N-({4-[(2-amino-6-ethyl-4-oxo-3,4-dihydrothieno[2,3-d]pyrimidin-5-yl)sulfanyl]phenyl}carbonyl)-L-glutamic 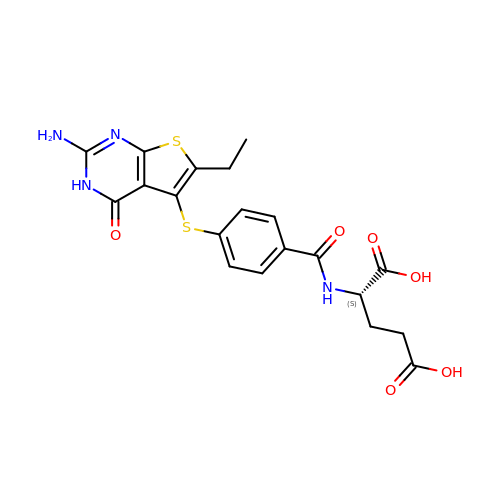acid | C20 H20 N4 O6 S2 | RSFXTHIRRXEJJD-NSHDSACASA-N> MGSNQSSSTSTKKLKAGNFDVAYQNPDKAIKGGNLKVAYQSDSPMKAQWLSGLSNDATFATMSGPGGGQDGLFFTDSGFKFIKGGAADVALDKESKTATITLRKDLKWSDGSEVTAKDYEFTYETIANPAYGSDRWTDSLANIVGLSDYHTGKAKTISGITFPDGENGKVIKVQFKEMKPGMTQSGNGYFLETVAPYQYLKDVAPKDLASSPKTTTKPLVTGPFKPENVVAGESIKYVPNPYYWGEKPKLNSITYEVVSTAKSVAALSSSKYDIINGMVSSQYKQVKNLKGYKVLGQQAMYISLMYYNLGHYDAKNSINVQDRKTPLQDQNVRQAI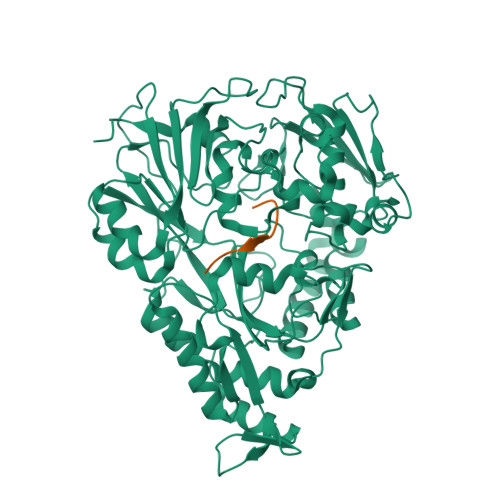GYARNVAEVDNKFSNGLSTPANSLIPPIFKQFTSSSVKGYEKQDLDKANKLLDEDGWKLNKSTGYREKDGKELSLVYAARVGDANAETIAQNYIQQWKKIGVKVSLYNGKLMEFNSWVDHMTTPPGANDWDITDGSWSLASEPSQQDLFSAAAPYNFGHFNDSEITKDLNDIDSAKSENPTYRKAAFVKYQEDMNKKAYVIPTNFMLNYTPVNKRVVGMTLDYGAMNTWSEIGVSSAKLATKGSIEGRHHHHHH;> SLSQSLSQS>[2x]MFKTEFEFPEELKTKLQEHINYFPKKRQAILLCLHEIQNYYGYIPPESLKPLADMLELPLNHVEGVVAFYDMFDREDKAKYRIRVCVSIVCHLMGTNKLLKALENILGIKPGEVTPDGKFKIVPVQCLGACSEAPVFMVNDDEYKFESEVQLNEILSRYT;>MRSYPAIPRIYAETTLNMLLKRAKKPRVHSIDEYLKDGGYQALEKALNMSPEEIIDWVDKSTLRGRGGAGFPTGKKWKFAVQNPGPRYFICNADEMEPGTFKDRIIIERDPHLLIEGIIISSYAIGANEAYIYIRGEYPAGYYILRDAIEEAKKKGFLGKNILGSGFDLEIYVARGAGAYICGEETALIESLEGKRGHPRLKPPYPVQKGLWGKPT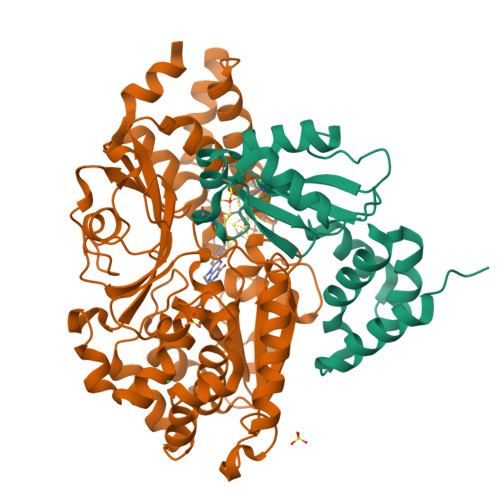VVNNVETIANVPFIISMGWEEYRYIGPSDYAGPKLFPVSGKVKKPGVYELPMNTTLREVIFKYAGGTLGNKKVKAVFSGALDCFSSEELDIPMDYSPLGFGGTGTVIVLTEEDDIVEAALKIAEFYEHETCGQCTPCRVGCYEQANLLEKIYKGEATEQDWEGFDFVNRNIQPTSICGLGAVAGRLIRQTLEKFPEEWEKYRKKSASLPLAGHHHHHH[2x]>GWNDPDRMLLRDVKALTLHYDRYTTSRRLDPIPQLKCVGGTAGCDSYTPKVIQCQNKGWDGYDVQWECCTDLDIAYKFGKTVVSCEGYESSEDQYVLRGSCGLEYNLDYTELGLQKLKESGKQHGFCSFSDYYYK[2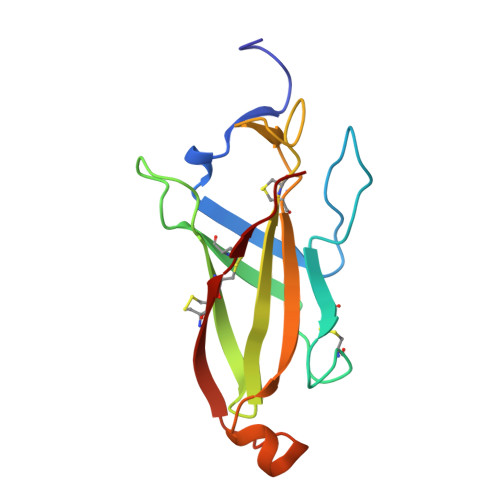x]>[2x]GSSGSSGNWIDVRYDLEKIESLIQSIHIDTTLY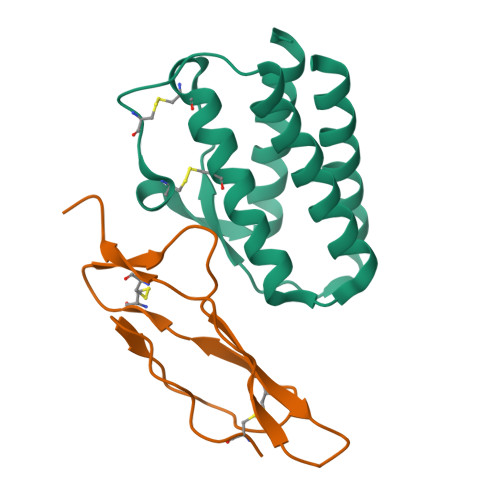TDSDFHPSCKVTAMNCFLLELQVILHEYSNMTLNETVRNVLYLANSTLSSNKNVAESGCKECEELEEKTFTEFLQSFIRIVQMFINTS;>GSSGSSGGTTCPPPVSIEHADIRVKNYSVNSRERYVCNSGFKRKAGTSTLIECVINKNTNVAHWTTPSLKCIRDPSLA[2x]> MKIERKFTTAEGGAYGGVGFTTTVSEIRNPDGTVVFRNESVEVPEGWSQVASDVLAQKYFRKAGVPARLKRVKEKGVPDFLWRSVPDEAELAKLPEEERFVGETSARQVFDRLAGAWAYWGWKGGYFSTEADARAYYDEMRHMLARQMAAPNSPQWFNTGLHWAYGIDGPSQGHFYVDHATGKLQKSDSAYEHPQPHACFIQSVQDDLVNEGGIMDLWVREARLFKYGSGTGTNFSSLRGEGEKLSGGGKSSGLMGFLKIGDRAAGAIKSGGTTRRAAKMVICDMDHPDIEQFINWKVIEEQKVASLVAGSKQHEAKLNDIFAAIRSFDGSIEGATDPAGNAGLKTAIRAAKKAMIPETYINRVLQYARQGFSSIEFPTYDTDWDSEAYTTVSGQNSNNSVRVTDAFLQAVKDDADWALVRRTDGKVAKTIKARELWDQVGHAAWACADPGIQFHDTVNAWHTCPEDGQIRGSNPCSEYMFLDDTACNLASMNLLTFFEAGRFDAEGYVHATRLWTVTLEISVMMAQFPSKEIAQLSYDFRT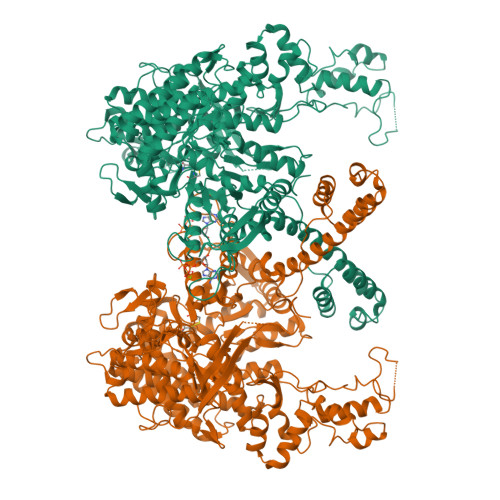LGLGYANIGGLLMNMGLGYDSSEGRALCGALSAIMTGVAYATSAEMAGELGAFSGYERNAGHMLRVIRNHRTAAHGHTTGYEGVNVSPVALDQVNCPDPRLVALAKSSWDEALRLGEAHGYRNAQVTVIAPTGTIGLVMDCDTTGIEPDFALVKFKKLAGGGYFKIINRSVPAALETLGYASAQISQIVAYAVGHGTLANCPTISHSALVGHGFGAREIEKIEAALPSAFDIRFVFNQWTLGEDFCKGALGIPADKLADPTFDLLRHLGFTRAQIEAANDHVCGTMTLEGAPHLKAEHLPVFDCANPCGKKGKRYLSVESHIHMMAAAQSFISGAISKTINMPNSATIAETLAAYELSHSLGIKANALYRDGSKLSQPLASAL>[6x]ASAKLPGDFGPPRGEPIHAVLTSPPLVPPPVNRTYPAKVIVELEVVEKEMQISEGVSYTFWTFGGTVPGSFIRVRQGDTVEFHLKNHPSSKMPHNIDLHGVTGPGGGAASSFTAPGHESQFTFKALNEGIYVYHCATAPVGMHIANGMYGLILVEPPEGLPKVDHEYYVMQGDFYTAGKYREKGLQPFDMEKAIDERPSYVLFNG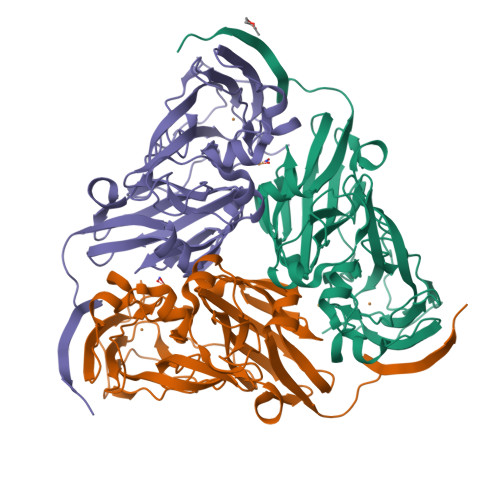AEGALTGDKALHAKVGETVRIFVGNGGPNLVSSFHVIGAIFDQVRYEGGTNVQKNVQTTLIPAGGAAVVKFTARVPGSYVLVDHSIFRAFNKGAMAILKIDGAENKLVYSGKELDSVYLGDRAAPN> MIEIFKDTGATHDLVYHSKINTFVWDVEFDIVLS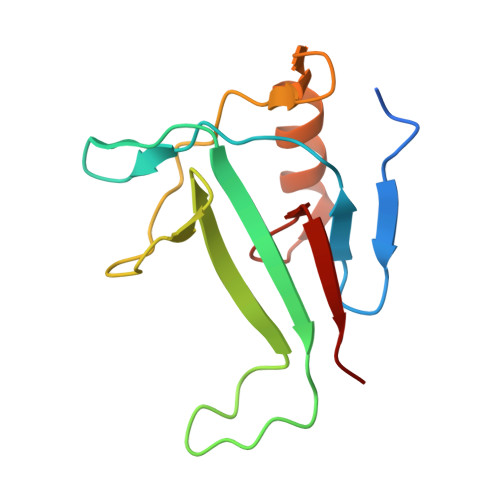DSKELNKCYFVKCFNPYRINGKCDFAVSSIDIFSEGKRLLIENEFNFKITKAVHVATSKDVTEIVLHLSERISSPFPIVKEVVYLD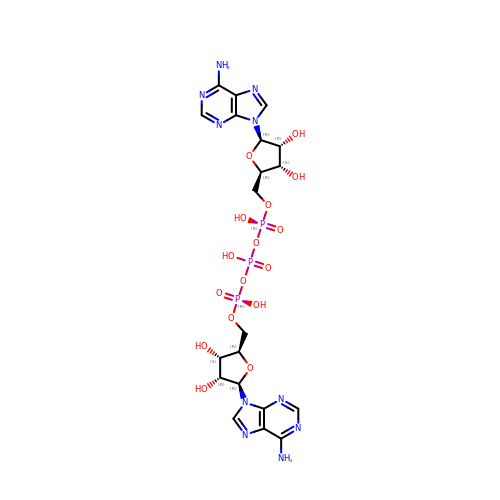BIS(ADENOSINE)-5'-TRIPHOSPHATE | C20 H27 N10 O16 P3 | QCICUPZZLIQAPA-XPWFQUROSA-N>[2x]GEELEYKGMNTLQISNVDDLISFYQYADDRIPLISGHRGGRGKGYPENSMETFENTLSYTPATFEIDPRLTKDSVIVLFHDDTLERTSNGTGKVSDYTWEELQNFRLKDPEGNITNYRIPTLEEAIRWARGKTILILDKKDVPMERTAQLITDMQAEPYVMITVHDGASARFFYEKNPNFMFEAFVKTKEAVQDYEDNGIPWSHIMAYVGPKITPEVREVIDMLHERGVMCMISTAP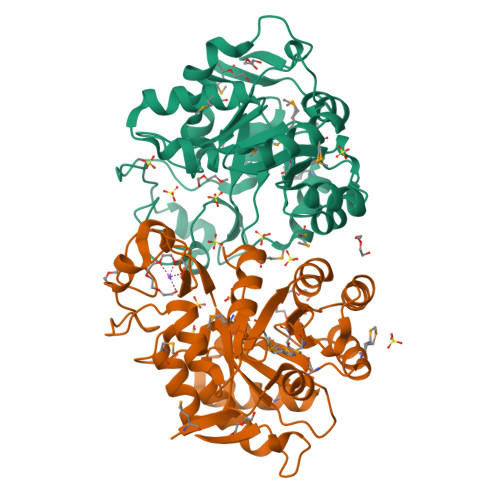SDDKLSTPESRAEAYRMIIRQGVDIIESDRPIEVAEAISSLIPVSSSKGKFFSTL>[2x]GSHMTDLAGPTITPNLQLVYVSNVERSTDFYRFIFKKEPVFVTPRYVAFPSSGDALFAIWSGGEEPVAEIPRFSEIGIMLPTGEDVDKLFNEWTKQKSHQIIVIKEPYTDVFGRTFLISDPDGHIIRVCPLD

Enterobacter agglomerans strain Eh1087 generates the phenazine antibiotic D-alanyl griseoluteic acid to compete with other microorganisms in its habitat. In order to protect itself against the toxic action of this compound, the bacterium produces the resistance protein EhpR together with enzymes required for phenazine biosynthesis. EhpR belongs to the glyoxalase I/bleomycin resistance protein family, whose members have a wide variety of functions extending from simple binding of toxic small molecules to their chemical conversion through enzymatic activity. The EhpR monomer consists of two βαββ'β fold units (' indicating antiparallel orientation with respect to the other strands) that are typical for members of the glyoxalase I/bleomycin resistance protein family.

In contrast to the apo structure, which crystallized with two EhpR dimers in the asymmetric unit, the asymmetric unit of GA-cocrystallized EhpR contains only one dimer despite having been obtained with the same precipitant. Data were collected to 1.01 Å and the final model has an R-factor or 12.6% with Rfree = 14.6%. In EhpR, the binding site adopts the shape of a cleft, and the interactions with GA involve hydrogen bonds between GA's carboxylate group and the side chains of R42 and W57 together with water-mediated contacts of the hydroxyl group with the side chain of Y43 and the carbonyl of L128* (* indicating residues of the second monomer). A large contribution to complex formation seemingly results from a π-stacking interaction of the phenazine ring system with the side chain of Y43. While the apo and complex structure are otherwise highly similar (average rmsd < 0.6 Å over the complete monomer), F109* undergoes a significant conformational and positional change on ligand binding. It adopts a different rotamer and moves together with the loop from E103 to G110, which leads to the formation of an open conformation of the ligand binding site with respect to the apo structure. Structural changes in the loop from E103 to G110 establish new crystal contacts, which explains the generation of a new crystal lattice in the cocrystallization experiment. Only one binding site was occupied in the structure obtained by cocrystallization. The other center remains blocked by the side chains of V108 and F109, which adopt the same conformation as in the apo structure here. The structure of EhpR in complex with griseoluteic acid suggests that it probably acts as a binder that works in tandem with a membrane-spanning exporter protein.>GQSITDYNYKKPLHNDYQILDKSKIF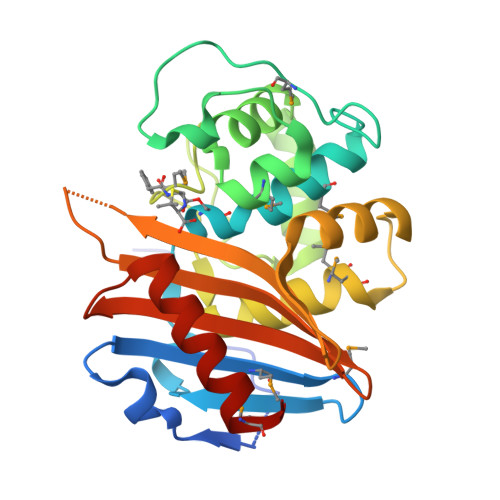GSNSGSFVMYSMKKDKYYIYNEKESRKRYSPNSTYKIYLAMFGLDRHIINDENSRMSWNHKHYPFDAWNKEQDLNTAMQNSVNWYFERISDQIPKNYTATQLKQLNYGNKNLGSYKSYWMEDSLKISNLEQVIVFKNMMEQNNHFSKKAKNQLSSSLLIKKNEKYELYGKTGTGIVNGKYNNGWFVGYVITNHDKYYFATHLSDGKPSGKNAELISEKILKEMGVLNGQ[2x]4-({4-amino-6-[4-(2-hydroxyethyl)-1H-imidazol-1-yl]pyrimidin-2-yl}amino)benzonitrile 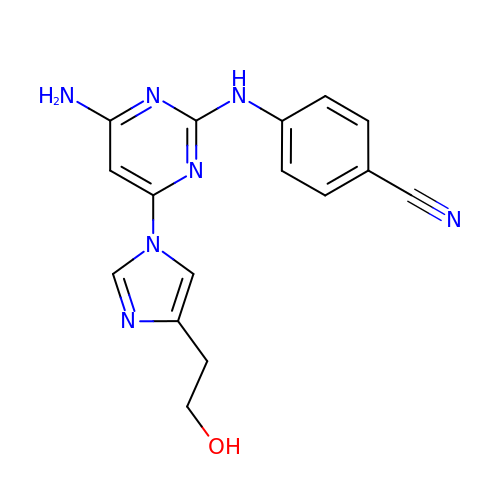| C16 H15 N7 O | OVFXXQZOTWTSJA-UHFFFAOYSA-N> MMRGIDSRHELDPTLLLRDTRTFTQRLADFFADPTNISIVLISLAAVSYYFSEAATFLLIMGGIFFLYSYTRKQKLPFRLPQISRAKDYNDLKPGINKPNIARGITFFGNDRKTGEELWFANDDMRTHALIFGSTGSGKTETLVSLSYNALVQGSGFIYVDGKGDNSLYAKVFSMVRSMGREDDLLLINFMTGARDIVGPQEKRLSNTLNPFCQGSSSMLTQLVVSLMGSSGQSSDGDMWKGRAIAFVEALMRLLVYMRDEGAILLDANTIRNYFDLQRLESIVIDKVFPRDDQESVNIETIPKLVTDPLRNYLNTLPGYNKEKKGKQVSQVLEQHGFITMQLVRSFSSLADTYGHIIRTNLAEVDFKDVVLNRRILVVLLPALEKSPDELSNLGKIIVSSLKAMMAAGLGEEVEGDYRDVILRKPTNAPTPYMCILDEYGYYAVQGFAVVPAQARSLGFSAIFAGQDLPAFQKASKEEAASIGANTNIKICMKLEDPTETWDFFTKTAGEAYVTKVDSFQTKETSIANSYMDTKSSSFEKRARVDLLDLKEQTEGEAHIFFKSKIVRARMFYANPKPVKQLKINQFLKVEPPPDDYLMKLQKQLASFQSILESGDLSINKAVENEEITLISKALKESTIVEPIERGVAALIAFHGQNEPEPVEDIVEEEVEGALTIFSKLRIDPNAPPILVADKEVFSEPLLPINETRNQMITIERLAGAKDKYAGTVANELIKDFQIATSYPPEERDVIDVQELTGIIRDLSAKISAEREKANKKAAEELT;> MYIEMAQQQQQSGSDNSMAPVWIVILLFITAYFVWALAHQYIVSFVFTINIWQARLVNLFLNNQLLANQIYLMQTLDPNTVNWDQMVTVMRAVGDYMRYPVICILVVLAFVLYNSNVTLKYRKTYDMKSLRAQEQFNWPAIMPIVKEDLVSQDVNKGPWAMALTPMEFARKYNLLRKDDALLDNPVPGEEMTAGIRRGDAKRVFTMQLGPYWDGFERCSPQAYALSAVFMARMNRDRDAANNILKVLDKTFVDGKPDFSVARPVMKKYQNSELVQEVVAKHAYVLTVIASLLEAAREDGVVPSSEFLWLKPVDRRLWYMLNCVGRQTPYSEVAGPFAHWKAEKEMGRRSLVPMIDEAIRALEIAVKEVRLTPRQMEELEP;> MADNQQRCELKLIASPGSWRLYSARKIDERFKSYEQKIFQRDRYTCQFCGFQARLYQDIVNLDGDYTNNRLSNLVTACCFCAQCFFVESVGVGGYGGGTLIYLPELTQAELNSLCHVLFCAITNDTGYKSSAQNIYRSFKFRSQIVEEKFGEGTSDPAIFGQLMIDSGVNSEEIREKLFKNIRLLPSRAKFRKQIEKWAASALEEIAD;> MDEIKKDDELSQWLSTYGTITAERILGRYNISLPQDEILEAINIPSSFYRHLLQIPLKNVLNGIVIQQASDYHVYAQKLLIDYLLSGESSKEPDSQGAGTRESLEDERQRLVQLGDEFHKLELEQDNLIASSQASLMKISIDWNTKLETTLSKLNSLYKNTNSKIKKNAIRKALIKAFIHCDLVKDQSQKNKYQLIDKLNQTLAVSVGAELKESILTNLSELFQILEALNTKLDEFTDRTNHLSQQAKSFRTQFYEVILRIIELIKLLPEYKIDPAQDAINREPLYFDRTIGER;> MPKYTLPTRDALLKAMQVGETSIEAAEYMATRFEQILTKAKLLPECNDMLEKIKEYAQFVKFKLLSSAQVWSGQERPTSDYQNTQENKAEFLASHLEGLPSGLKLEVAIGDDAKILRGFSSNGKMVEGDQLKTMDGLLEGWLAKNSLAISGGAVVKIDNTGNQTKVDPQEIRQLINDSEKGVAKYFADKGVGMEVAQRTYQEPKALETKREEIRQEIESGAEAPTTQSIR

The T4BSS is a complex nanomachine made up of several sub‐complexes, one of which, called the Type IV Coupling Complex (T4CC), has the primary function of recruiting effectors and delivering them to the trans‐membrane machinery for translocation into host cells. Integrated into the inner membrane, the T4CC is a multiprotein effector recruitment platform comprising different effector binding sites and an AAA+ ATPase called DotL. The structure revealed that the T4CC is made of two parts linked by the C‐terminal tail of DotL (DotLCter): the hetero‐pentameric core composed of the DotL ATPase domain, DotM, DotN, DotY, and DotZ (referred to as “DotLMNYZ core”), and the flexible IcmSW module composed of IcmS and IcmW (Kwak et al., 2017; Meir et al., 2020; Vincent et al., 2012). Finally, the T4CC contains at least two binding sites for recruitment of two different classes of effectors: one on DotM, proximal to a cavity at the center of the hetero‐pentameric core (Meir et al., 2018), and the second on the IcmSW module (Cambronne & Roy, 2007; Sutherland et al., 2012).

Here, we further investigate the function of DotY and DotZ proteins. First, we obtained a near‐atomic resolution cryo‐EM map that includes the middle domain of DotY previously missing. In the T4CC structure, DotY interacts exclusively with DotZ, which would explain why DotY would depend on DotZ to co‐purify with the other T4CC components. On the other hand, the dependence of the DotZ protein on DotY interaction with T4CC components is unexpected, because DotZ makes intensive interactions with DotLCter, DotM, and DotN. One potential explanation for this observation is that DotY stabilizes DotZ prior to assembly, allowing it to assume a conformation conducive to association with other T4CC components. For DotZ, residues at the interface with other T4CC component are conserved, while residues facing the cytoplasm are not. For DotY, most residues are not conserved. DALI (Holm, 2020) analysis shows that DotY and DotZ do not belong to any structural or functional family. The facts that DotY and DotZ are not essential for secretion, unique to the Legionella genus, located at the periphery of the complex, do not belong to any known structural and functional families, and poorly conserved suggest that DotY and DotZ have only recently been evolved to play a part in type IV secretion in Legionella. Further analysis reveals that the trajectory of the IcmSW module is modified by DotY/Z, thereby suggesting the likely function of these proteins.>[2x]MIEWQDLHHSELSVSQLYALLQLRCAVFVVEQNCPYQDIDGDDLTG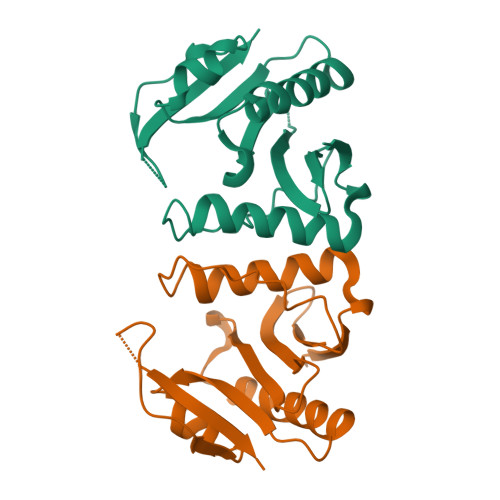DNRHILGWKNDELVAYARILKSDDDLEPVVIGRVIVSEALRGEKVGQQLMSKTLETCTHHWPDKPVYLGAQAHLQNFYQSFGFIPVTEVYEEDGIPHIGMAREVIQA>MHHHHHHTMGGSVDGQGLLQLDKDTFWPYLEQQQDTLVVVDFYTDWCGPCKLIYPELVKLSQERTDVRFVKVNCNKSNKELGMQLAIKVAPTFHLYRNKTKVADMTGAKMDKLIALINQHQPPKN[3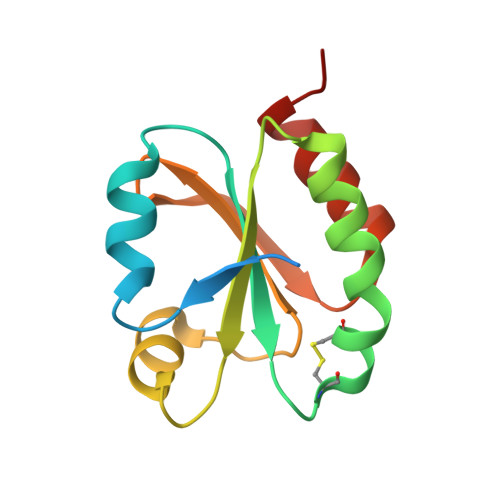x]Here, we report the in situ near-atomic resolution structures of RdRp before and during transcription in rotavirus double layered particles (DLP). The RdRp has a conserved hand-shaped core domain (residues 333–778), which is sandwiched between an N-terminal domain (residues 1–332) and a C-terminal domain (residues 779–1088). This core domain can further be divided into the fingers, palm, and thumb subdomains, with the active site located between the fingers and palm. An atomic model was built based on this high-resolution in situ structure, with distinct side chain densities and RNA features. We determined that the RdRp is attached to CSP decamers at a specific, off-centered location, as previously described.

To further study conservative transcriptional mechanisms, we imaged DLPs at non-transcribing state with the same methods. In the final sub-particle reconstruction at 3.4 Å resolution, we found no RNA density in the active site; however, two ssRNAs that attach to two separate positions on the surface of RdRp were detected. As detailed below, we interpret that these two ssRNAs are the result of an open genomic duplex. Thus, the RdRps in these DLPs existed mainly in a duplex-open state (DOS) compared to TES. In DOS, the cap-binding site of the N-terminal domain in RdRp interacts with the conserved terminal m7G(5′)ppp(5′)GGC residues of the genomic (+) strand in all segments of the rotavirus genome. Compared with other resolved reovirus RdRp structures, the rotavirus RdRp’ N-terminal domain possesses an additional subdomain that has a helix-loop-helix structural feature (residues 31–69, HLH subdomain) near the cap-binding site. This HLH subdomain extends towards the genomic (+) strand in DOS and retracts from RNA in TES. In DOS, the (−)RNA weakly interacts with an ssRNA-binding β-sheet subdomain (residues 400–419) in the fingers (residues 333–488, 524–595) of the core, which can bind ssRNA both specifically and nonspecifically. In DOS, however, the C-HB subdomain retracts from CSP-A1 and narrows the transcript exit channel, such that CSP-A1 returns to a similar conformation as the ones found in CSP-A3–5. However, the corresponding amphipathic helix in CSP-A4 attaches to the C-HB of RdRp in DOS and detaches from RdRp in TES. A unique C-terminal plug (residues 1072–1088) inserts into the template exit channel in DOS, but moves away in TES to allow (−)RNA to exit.

> MGKYNLILSEYLSFIYNSQSAVQIPIYYSSNSELENRCIEFHSKCLENSKNGLSLKKLFVEYSDVIENATLLSILSYSYDKYNAVERKLVKYAKGKPLEADLTVNELDYENNKITSELFPTAEEYTDLLMDPAILTSLSSNLNAVMFWLEKHENDVAEKLKIYKRRLDLFTIVASTVNKYGVPRHNAKYRYEYEVMKDKPYYLVTWANSSIEMLMSVFSHEDYLIARELIVLSYSNRSTLAKLVSSPMSILVALVDINGTFITNEELELEFSNKYVRAIVPDQTFDELKQMLDNMRKAGLTDIPKMIQDWLVDCSIEKFPLMAKIYSWSFHVGFRKQKMLDAALDQLKTEYTEDVDDEMYREYTMLIRDEVVKMLEEPVKHDDHLLQDSELAGLLSMSSASNGESRQLKFGRKTIFSTKKNMHVMDDMANGRYTPGIIPPVNVDKPIPLGRRDVPGRRTRIIFILPYEYFIAQHAVVEKMLIYAKHTREYAEFYSQSNQLLSYGDVTRFLSNNSMVLYTDVSQWDSSQHNTQPFRKGIIMGLDMLANMTNDARVIQTLNLYKQTQINLMDSYVQIPDGNVIKKIQYGAVASGEKQTKAANSIANLALIKTVLSRISNKYSFATKIIRVDGDDNYAVLQFNTEVTKQMVQDVSNDVRETYARMNTKVKALVSTVGIEIAKRYIAGGKIFFRAGINLLNNEKKGQSTQWDQAAVLYSNYIVNRLRGFETDREFILTKIMQMTSVAITGSLRLFPSERVLTTNSTFKVFDSEDFIIEYGTTDDEVYIQRAFMSLSSQKSGIADEIAASSTFKNYVSRLSEQLLFSKNNIVSRGIALTEKAKLNSYAPISLEKRRAQISALLTMLQKPVTFKSSKITINDILRDIKPFFTVNEAHLPIQYQKFMPTLPDNVQYIIQCIGSRTYQIEDDGSKSAISRLISKYSVYKPSIEELYKVISLHENEIQLYLISLGIPKIDADTYVGSKIYSQDKYRILESYVYNLLSINYGCYQLFDFNSPDLEKLIRIPFKGKIPAVTFILHLYAKLEVINHAIKNGSWISLFCNYPKSEMIKLWKKMWNITSLRSPYTNANFFQD;>[10x]MAYRKRGARRETNLKQDDRMQEKEENKNVNTNSENKNATKPQLSEKVLSQKEEVITDNQEEIKIADEVKKSNKEESKQLLEVLKTKEEHQKEVQYEILQKTIPTFEPKESILKKLEDIKPEQVKKQTKLFRIFEPRQLPVYRANGEKELRNRWYWKLKRDTLPDGDYDVREYFLNLYDQVLTEMPDYLLLKDMAVENKNSRDAGKVVDSETAAICDAIFQDEETEGVVRRFIAEMRQRVQADRNVVNYPSILHPIDHAFNEYFLQHQLVEPLNNDIIFNYIPERIRNDVNYILNMDRNLPSTARYIRPNLLQDRLNLHDNFESLWDTITTSNYILARSVVPDLKELVSTEAQIQKMSQDLQLEALTIQSETQFLTGINSQAANDCFKTLIAAMLSQRTMSLDFVTTNYMSLISGMWLLTVVPNDMFIRESLVACQLAIINTIIYPAFGMQRMHYRNGDPQTPFQIAEQQIQNFQVANWLHFVNNNQFRQVVIDGVLNQVLNDNIRNGHVVNQLMEALMQLSRQQFPTMPVDYKRSIQRGILLLSNRLGQLVDLTRLLAYNYETLMACITMNMQHVQTLTTEKLQLTSVTSLCMLIGNATVIPSPQTLFHYYNVNVNFHSNYNERINDAVAIITAANRLNLYQKKMKSIVEDFLKRLQIFDISRVPDDQMYRLRDRLRLLPVEIRRLDIFNLILMNMEQIERASDKIAQGVIIAYRDMQLERDEMYGYVNIARNLDGFQQINLEELMRTGDYAQITNMLLNNQPVALVGALPFITDSSVISLVAKLDATVFAQIVKLRKVDTLKPILYKINSDSNDFYLVANYDWVPTSTTKVYKQIPQQFDFRASMHMLTSNLTFTVYSDLLAFVSADTVEPINAVAFDNMRIMNEL>[4x]GPLIKENMRMKVV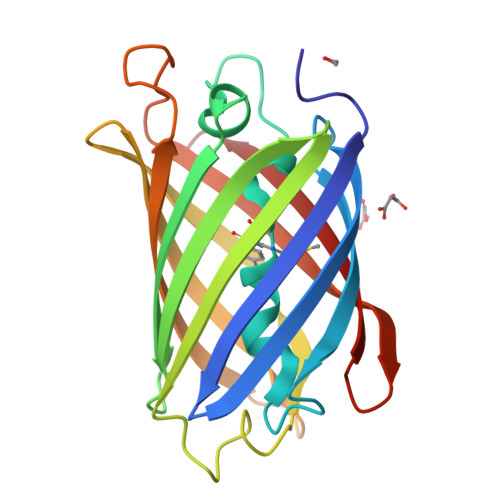MEGSVNGHQFKCTGEGEGRPYEGVQTMRIKVIEGGPLPFAFDILATSFMYGSRTFIKYPADIPDFFKQSFPEGFTWERVTRYEDGGVVTVTQDTSLEDGELVYNVKVRGVNFPSNGPVMQKKTKGWEADTEMMYPADGGLRGYLDRALKVDGGGHLHCNFVTTYRSKKTVGDIKMPGVHAVDHRLERIEESDNETYVVQREVAVAKYS>SAHPWKAPGPNDSRGPCPGLNTLANHGFLPRNGRNISVPMIVKAGFEGYNVQSDILILAGKIGMLTSREADTISLEDLKLHGTIEHDASLSREDVAIGDNLHFNEAIFTTLANSNPGADVYNISSAAQVQHDRLADSLARNPNVTNTDLTATIRSSESAFFLTVMSAGDPLRGEAPKKFVNVFF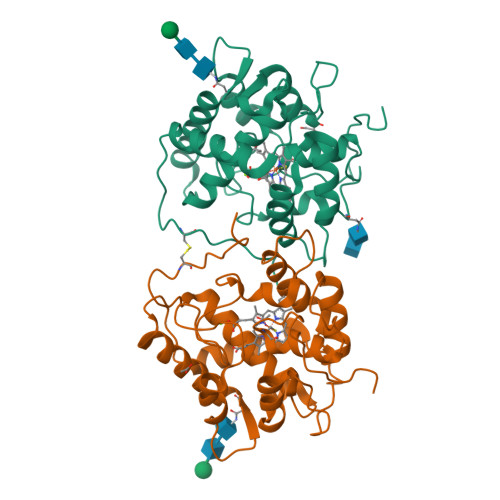REERMPIKEGWKRSTTPITIPLLGPIIERITELSDWKPTGDNCGAIVLSPEL[2x]(2R)-4-(1,3-dioxo-1,3-dihydro-2H-isoindol-2-yl)-N-hydroxy-2-{[(4'-methoxybiphenyl-4-yl)sulfonyl](propan-2-yloxy)amino}butanamide | C28 H29 N3 O8 S 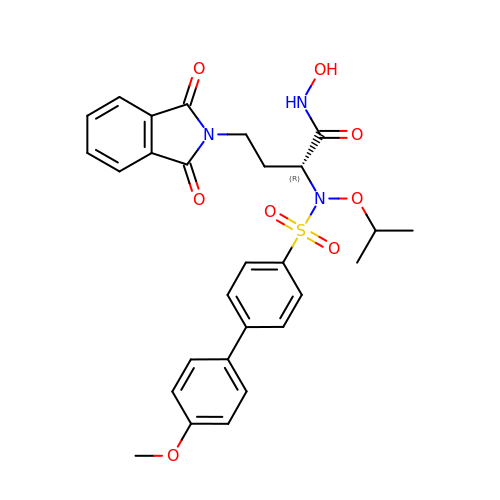| WQCXDERWRJMJQA-RUZDIDTESA-N> SKLKDPELSLKGTQHIMQAGQT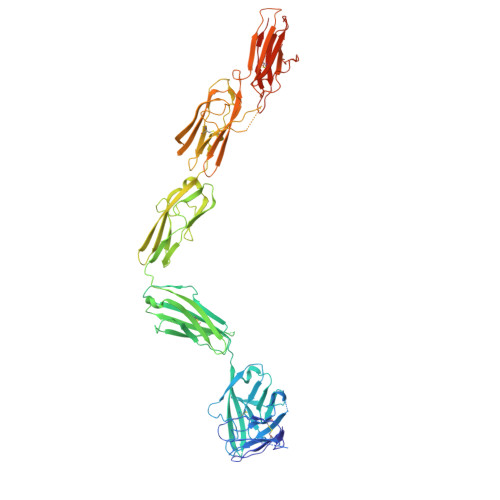LHLQCRGEAAHKWSLPEMVSKESERLSITKSACGRNGKQFCSTLTLNTAQANHTGFYSCKYLAVPTSKKKETESAIYIFISDTGRPFVEMYSEIPEIIHMTEGRELVIPCRVTSPNITVTLKKFPLDTLIPDGKRIIWDSRKGFIISNATYKEIGLLTCEATVNGHLYKTNYLTHRQTNTIIDVQISTPRPVKLLRGHTLVLNCTATTPLNTRVQMTWSYPDEKNKRASVRRRIDQSNSHANIFYSVLTIDKMQNKDKGLYTCRVRSGPSFKSVNTSVHIYDKAFITVKHRKQQVLETVAGKRSYRLSMKVKAFPSPEVVWLKDGLPATEKSARYLTRGYSLIIKDVTEEDAGNYTILLSIKQSNVFKNLTATLIVNVKPQIYEKAVSSFPDPALYPLGSRQILTCTAYGIPQPTIKWFWHPCNHNHSEARCDFCSNNEESFILDADSNMGNRIESITQRMAIIEGKNKMASTLVVADSRISGIYICIASNKVGTVGRNISFYITDVPNGFHVNLEKMPTEGEDLKLSCTVNKFLYRDVTWILLRTVNNRTMHYSISKQKMAITKEHSITLNLTIMNVSLQDSGTYACRARNVYTGEEILQKKEITIRDQEAIEGRHHHHHHHH>[2x]NYMGNPWTEYMAKYDIEEVHGSGIRVDLGEDAEVAGTQYRLPSGKCPVFGKGIIIENSNTTFLTPVATGNQYLKDGGFAFPPTEPLMSPMTLDEMRHFYKDNKYVKNLDELTLCSRHAGNMIPDNDKNSNYKYPAVYDDKDKKCHILYIAAQENNGPRYCNKDESKRNSMFCFRPAKDISFQNYTYLS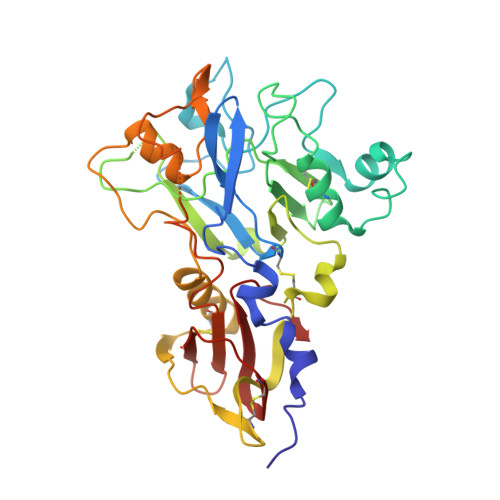KNVVDNWEKVCPRKNLQNAKFGLWVDGNCEDIPHVNEFPAIDLFECNKLVFELSASDQPKQYEQHLTDYEKIKEGFKNKNASMIKSAFLPTGAFKADRYKSHGKGYNWGNYNTETQKCEIFNVKPTCLINNSSYIATTALSHPIEVE>LQFYRNLGKSGLRVSCLGLGTWVTFGGQITDEMAEHLMTLAYDNGINLFDTAEVYAAGKAEVVLGNIIKKKGWRRSSLVITTKIFWGGKAETERGLSRKHIIEGLKASLERLQLEYVDVVFANRPDPNTPMEETVRAMTHVINQGM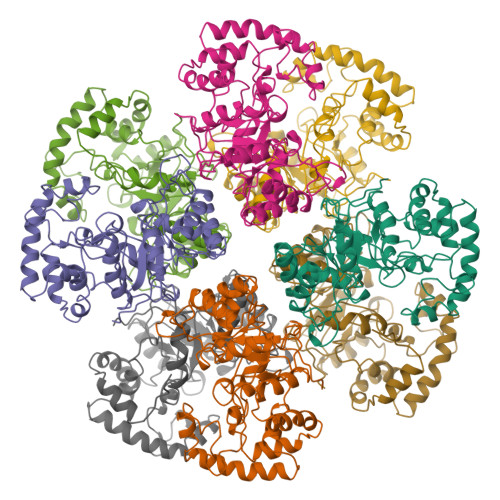AMYWGTSRWSSMEIMEAYSVARQFNLIPPICEQAEYHMFQREKVEVQLPELFHKIGVGAMTWSPLACGIVSGKYDSGIPPYSRASLKGYQWLKDKILSEEGRRQQAKLKELQAIAERLGCTLPQLAIAWCLRNEGVSSVLLGASNAEQLMENIGAIQVLPKLSSSIVHEIDSILGNKPYS[8x]> MEQLTKCEVFQKLKDLKDYGGVSLPEWVCVAFHTSGYDTQAIVQNNDSTEYGLFQINNKIWCKDDQNPHSRNICNISCDKFLDDDLTDDIVCAKKILDKVGINYWLAHKALCSEKLDQWLC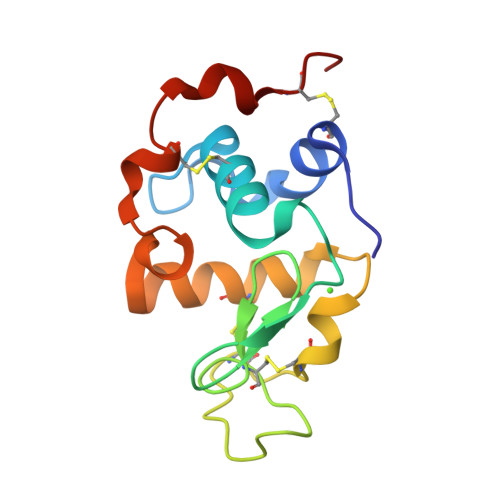EKL Enolase (2-phospho-d-glycerate hydrolyase, EC 4.2.1.11) catalyzes the conversion of 2-phosphoglycerate (2-PGA) to phosphoenolpyruvate (PEP) during both glycolysis and gluconeogenesis in all three domains of life. Enolase is a metalloenzyme activated by cations of bivalent metals, such as magnesium (Mg2+). In the present study, we purified enolase-1 from Chloroflexus aurantiacus (EnoCa), a thermophilic green non-sulfur bacterium that grows photosynthetically under anaerobic conditions. Each monomer of EnoCa contains an amino terminal domain that consists of a three-stranded β-sheet packed against three α-helices and a carboxy terminal domain that consists of an eightfold α/β-barrel; both domain features are typical of the enolase superfamily.

High-resolution crystal structures were obtained for the apo protein as well as proteins with 2-PGA and PEP bound in the active site. The EnoCa structure containing PEP (PEP EnoCa structure) exhibits the so-called “closed” conformation, where the L1 loop is located closer to the active site. Like the apo EnoCa structure, a metal ion was mapped to the active site in the 2-PGA and PEP structures. The presence of 2-PGA and PEP in the active site of EnoCa was confirmed by calculation of a simulated-annealing OMIT map. In contrast to the 2-PGA EnoCa structure, PEP was coordinated with the second catalytic metal atom in the active site. The second atom was identified as Mg2+. Mg2+(II) was coordinated with Ser43, water molecules, and phosphate atoms from PEP supporting the octahedral coordination sphere. PEP itself is bound by Glu165, Glu206, Lys338, Arg367, and Ser368. It should be noted that the electron density was absent for the Ser43 in subunit A of the PEP EnoCa structure due to instability of the L1 region. Nevertheless, the Ser43 was modeled in subunit A with reduced occupancy (0.5).

>MSTLIEAIVAREVLDSRGNPTIEVDVRLESGDVGRAIVPSGASTGAHEALELRDGDKSRYNGKGVLKAVQAVNEDIAEALIGFDAADQIALDQELIALDGTPNKSKLGANAILGVSLAAAKAAAAAFGLPLYRYLGGVYAHVLPVPMMNIMNGGQHATNSTDFQEFMIMPVGAESFREGLRWGAEIYHMLKKVIHDRGFSTTVGDEGGFAPSLPTNDAPLQLIMEAIEKAGYRPGEQIVIALDPATTEIFEDGKYHLKREGRSLSSAEMVDYWVDLVNRYPIISLEDGLAEDDWEGWALLRAKLGDRVQLVGDDFLVTNVQRLQRAIEAKAANSILIKLNQIGSLTETLSAIQLAQRSGWTAVVSHRSGESEDVTIADLVVATNAGQIKTGAPARTDRIAKYNQLLRIEEELGSAARYAGRSAFKV[2x]>[5x]KYIPRIAEDMTIQEAKKFARENNIKEGKIDEIMHDSIQDTAEQKVQLLLCWYQSHGKSDAYQDLIKGLKKAECRRTLDKFQDMVQK;>[5x]GEEDLCAAFNVICDNVGK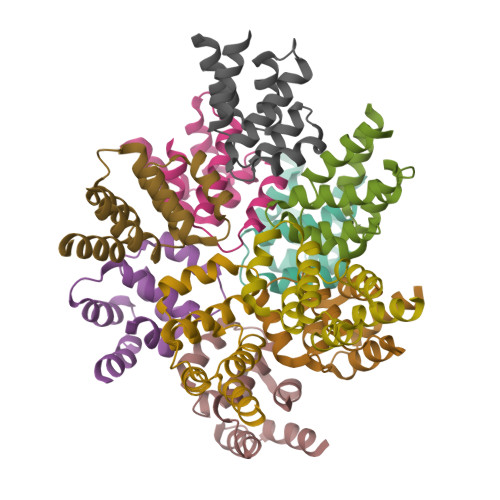DWRRLARQLKVSDTKIDSIEDRYPRNLTERVRESLRIWKNTEKENATVAHLVGALRSCQMNLVADLVQEVQQARLEHHHHHH> GSMDITRFKEDLKAHLEEKIIPFWQSLKDDEFGGYYGYMDFNLNIDRKAQKGCILNSRILWFFSACYNVLKSEKCKEMAFHAFEFLKNKFWDKEYEGLFWSVSHKGVPVDVTKHVYVQAFGIYGLSEYYEASGDEEALHMAKRLFEILETKCKRENGYTEQFERNWQEKENRFLSE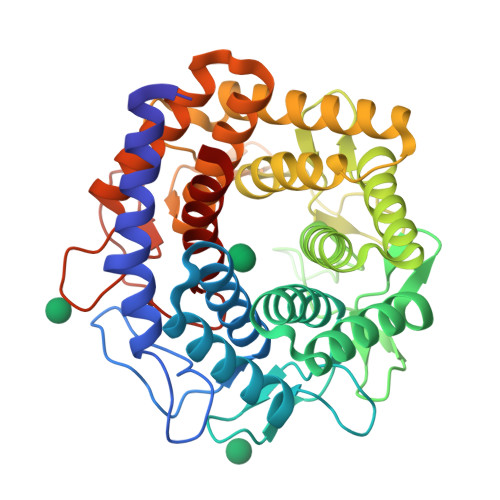NGVIASKTMNTHLHVLESYTNLYRLLKLDDVYEALEWIVRLFVDKIYKKGTGHFKVFCDDNWNELIKAVSYGFDIEASWLLDQAAKYLKDEKLKEEVEKLALEVAQITLKEAFDGQSLINEMIEDRIDRSKIWWVEAETVVGFFNAYQKTKEEKYLDAAIKTWEFIKEHLVDRRKNSEWLWKVNEDLEAVNMPIVEQWKCPYHNGRMCLEIIKRV>[15x]DSLKWIVFLLFLI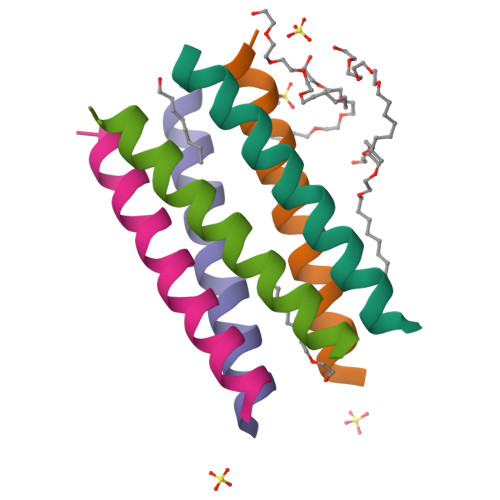VLLLLAIVFLLRGX1-(5-tert-butyl-1,2-oxazol-3-yl)-3-(4-{7-[2-(morpholin-4-yl)ethoxy]imidazo[2,1-b][1,3]benzothiazol-2-yl}phenyl)urea 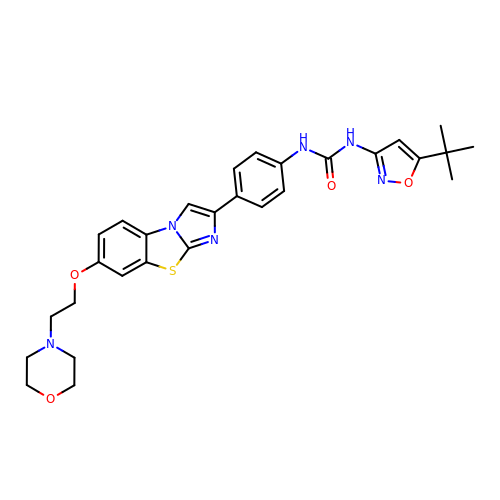| C29 H32 N6 O4 S | CVWXJKQAOSCOAB-UHFFFAOYSA-N> SNAACSTSGGDKKTSTNSSSGGDSKSEEKLAAKQVFNKTENQEIPTMDTSKSTDTLGSQILGNTMEGLYRLDKENKPIPAAAESSTKSEDGKKYTFKLRKDAKWSNGDSVTAKDFVFAWQRLLDPKTAAEYAFIAFPIKNAEAV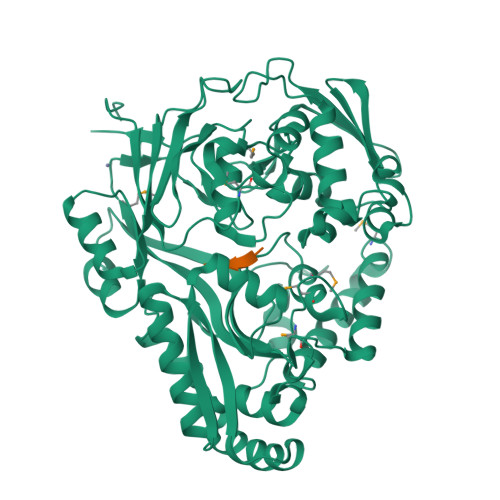NKGEKPVTELGVKAVDDLTLEVELEQAVPYFLNLVAFPSYYPLNEKFVKEKGDKYGLESDTTVYNGPFVLTDWKHEQGWKLKKNDQYWDKKTVKLDEINYSVVKEPATNVNLYDSGQIDFSLLTGEFVDKYRNNKEEYGVYNEPSTFFIRLNQKRGGQDTPLKSKKLREAIALSIDKKNLTNVILNDGSKPADYLVPKGLAAGPDGKDFQETFKNGVKPDAKKAAAAWEEAKKELGKDQVTIEFLNYDTGNAKKVGEYVKDQIEKNLKGVTVNIKLQPFKQKLKLESDQDYDISYGGWSPDYADPMTYLDMFESKHSHNQMSFSDQKYDEIIKKAGGELMTDAKKRWEELGKAEELLLEEDVALVPLYQSARSYVMKPHVKGVVKHNISPEYSYKWAYVTEK> MSAIKPDMKIKLRMEGNVNGHHFVIDGDGTGKPFEGKQSMDLEVKEGGPLPFAFDILTTAFLYGNRVFAKYPDNIQDYFKQSFPKGYSWERSLTFEDGGICNARNDITM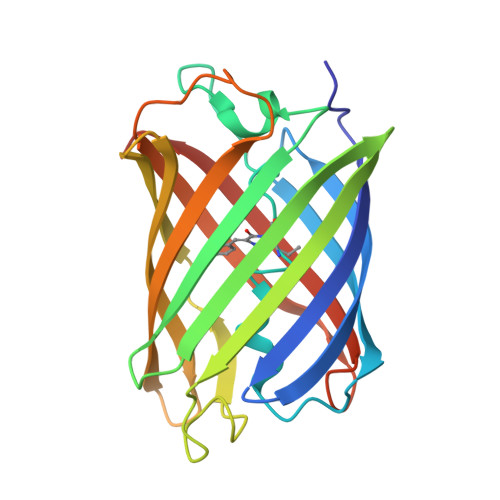EGDTFYNKVRFYGTNFPANGPVMQKKTLKWEPSTEKMYVRDGVLTGDVEMALLLEGNAHYRCDFRTTYKAKEKGVKLPGAHFVDHCIEILSHDKDYNKVKLYEHAVAHSGLPDNARR>MAARRFCVGGNWKMHGSKNSIRDICNTLKGASLDPNVEVIVACPAPYLDYCRSLLPPSVALAAQNCYKVEQGAFTGEISPGMIKDCGGQWVILGHSERRHVFKEDDVLIGEKIKHALESGLNVIACIGEL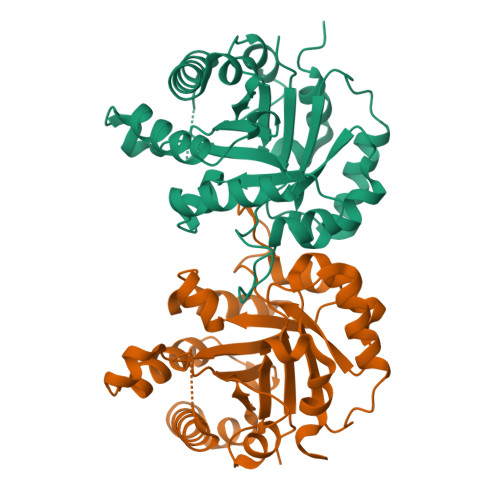LEDREAGRTEEVCFRQIKHIASNVKDWSKVVIAYEPVWAIGTGKTATPDQAQEVHSKVRNWLSTNVSADVASKVRIQYGGSVNAGNCKELGRKPDIDGFLVGGASLKPEFVQIINAMQG[2x]Cypoviruses, members of the family Reoviridae, subfamily Spinareovirus, possess a single capsid layer with turrets and are commonly embedded in crystalline occlusion bodies called polyhedra, which are formed in the cell cytoplasm and mainly composed of a single virus-encoded protein, polyhedrin. To ensure the delivery of virus particles to the target intestinal cells, allowing the transmission of packages of infectious virus between hosts by oral-faecal routes, polyhedra are disrupted only when they are exposed to the very alkaline pH environment found in insect midguts. The fold of all the polyhedrins is highly similar – a β-barrel core sitting on a base domain, surrounded by a common array of five helices (H1–H5). The strongest intermolecular interactions define a trimer composed of a cluster of three β-barrels sandwiched by helices top and bottom.

CPV4 features long V1 and V5, which loop back to interact. All polyhedra belong to the same I23 space group and the native crystals (at 100 K) mostly possess a unit cell of 102–103 Å (102.8 ± 0.4 Å). The exceptions were CPV4, which forms crystals with 2 distinct unit cell dimensions (101.7 and 104.8 Å – the structure of the larger unit cell is an outlier and is discussed below), and CPV17 which has larger cell dimensions (106.1 Å room temperature and 104.9 Å 100 K). Native crystals of CPV4 polyhedra grouped into two distinct unit cell dimensions, 101.7 (±0.27) Å and 104.8 (±0.18) Å, whilst all SeMet crystals had the larger size. Crystals with both unit cell dimensions were observed on each of several frozen meshes suggesting that this was not an artefact of sample preparation. Thus in CPV4, the purines are replaced by greatly elongated V1 and V5 regions, whilst the shortened V4 loop would no longer be able to contact the ATP. CPV4 has limited numbers of molecular interactions in this area, while in CPV5 a few strong trimer-trimer interactions are present. In CPV1, 14, 15, 17, 18 and 20 solvent molecules can move between these two voids, whereas in CPV4, 5 and 19 they are blocked by tyrosine residues.

> XSTSTYALRAGKRDVRREQQEIITRQINTAPYVQDAMMRVVVFAQYPSGRYKAFDYVFPDYLKVFLNWRELLEDTTTDYDPRTNTHRLMGQGYRQLIHPNHGSGEEPYDTRYPMGVIVSFNGNIDWTRARVEATNMHGLNNTDWREARAWGPHVICGNQLRKAGHLSRAVYVPLDEHNTVKVLATARQDGALNRFNGPQLAQTLTNNIVCPNVIEFNTESDVIDYAKMAHIAYIDQAGLIVASSDAYISGDSQA> GPGSMAAGTQVIANSGHDDMIHDAVLDYYGRRLATCSSDRTIKIFEIEGETQRLTETLKGHDGAVWCVSWAHPKYGNILASAGYDGKVLI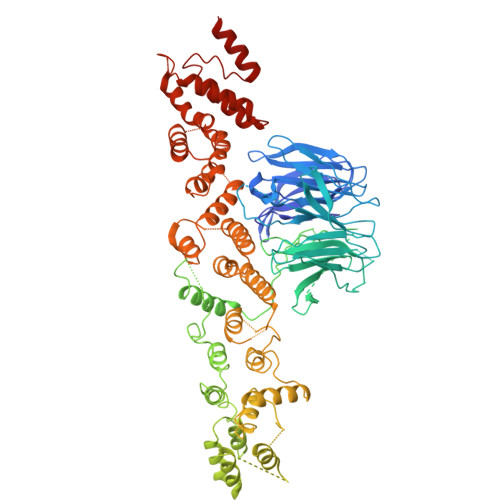WRELNGAWQRIFDFALHKASVNVVSWSPHEAGCLLACASSDGNVSVLEFRDNSWEHSIFHAHGLGVNSVSWAPATSPGSIVSSKPGPKSTGNRRFVTGGSDNALKIWAYDPATNTYKLEREPLTGHTDWVRDVAWSPTVLQKSYIASASEDRTVRIWTSDPANPLQWNCKVLNFDAAVWRVSWSLSGNVLAASGGDNKVTLWKENLKGEWECVKTIEEGGGGSGGGGQAKGPTQPEQASPAKGFVKWPYQQRPKIDQQEGPSIPRTNWGPNGLLVTTHHGEPSLQPADGTLAASEESVGSPENLARLQRYIDSVSFKEGQPIASPEFRELAQGDPSWELASLLFDDNGYGLPAFWRQLVSEATDRALAQEPGLEEKAIICLAGNRVADACGYLLAAGNFRLATLVSGIGMQDGDMKAQLKDWRESNVLAEFSQPVRAIYELLAGNAGVCAGVKNVPIENRVDSFTISQRFGLDWMRSFGLRLFYTTGATANVAEAVRSFQADIEQDKEPEPDSALWSLLKAFANQEFDWSDTRLGWLLTKAIYATGKVSFGQDAAEKLDKASLAYASALTAQSQWVPATFVLLQLSDAASREAAVRDHLGRHARRIGSPRNPNSAFSSLRKFGVPETWIWEAKALDFRARGDSQQEFLALVWAQNYSEANQAFVHRVGPDLVIARDFRRLFRFAQLLFKVKGKLQDWDRGAAVYLLYPMARLQGKQHGLDKFDHQLFDGLVALRGQTHGDIRQEAAIADMAEDLIRCRGGDPRLFGLLPEDVRSKYMRAQALEVIC> SLGIFPTVEKLVEEMREQLDEVDSHPRTSIFEKLPSKRDYPDYFKVIEKPMAIDIILKNCKNGTYKTLEEVRQALQTMFENARFYNEEGSWVYVDADKLNEFTDEWFKEHSS;> TARKSTGGKAPRKQLASY

Lysine benzoylation (Kbz) is a recently discovered post-translational modification associated with active transcription. Here, we systematically characterize writer, eraser, and reader proteins of histone Kbz in S. cerevisiae using proteomic, biochemical, and structural approaches. The Spt-Ada-Gcn5 acetyltransferase (SAGA) complex and NAD+-dependent histone deacetylase Hst2 could function as the writer and eraser of histone Kbz, respectively. In addition, we demonstrate that a subset of YEATS domains and bromodomains serve as Kbz readers, and structural analyses reveal how YEATS and bromodomains recognize Kbz marks.

There are 15 bromodomains in S. cerevisiae, and we purified four of these bromodomains and characterized their binding abilities with H3K14bz and H3K27bz peptides. Although most bromodomains showed negligible H3K14bz or H3K27bz binding abilities, the Bromodomain from Sth1 (Sth1BD), the ATPase subunit in the Remodel the Structure of Chromatin (RSC) complex, surprisingly exhibited robust interaction with H3K14bz (Kd = 89 μM), albeit weaker than that with H3K14ac (Kd = 16 μM)36 Fig. 6 Sth1 bromodomain has Kbz binding activity. To reveal how Sth1BD recognizes Kbz, we determined the crystal structure of Sth1BD in the complex with the H3K14bz peptide at a resolution of 1.4 Å. The H3 peptide is well ordered, as evidenced by good electron density from T6 to Y23. Histone H3 sits on the acidic apical region of the Sth1BD helical bundle and makes extensive contacts with the ZA-loop, BC-loop, αZ′, αA′, αB, and αC of Sth1BD. The overall complex conformation is highly similar to that of Sth1BD-H3K14ac, except for the shift of the H3 C-terminal 310-helix (K18-A21). The indistinguishable configurations of the Kbz- and Kac-binding pockets indicate that the acylation-binding pocket of Sth1BD intrinsically has adequate space to accommodate the large benzene ring without any structural rearrangement. The Sth1BD-H3K14bz structure clearly shows that the acylation-binding pocket of Sth1 has adequate space to accommodate the large benzene ring without any structural rearrangement of Sth1BD. This indicates that although most bromodomains have small acyl-binding pockets suitable for short acetyl marks, certain bromodomains can bind diverse acylation marks other than acetylation.>PPGP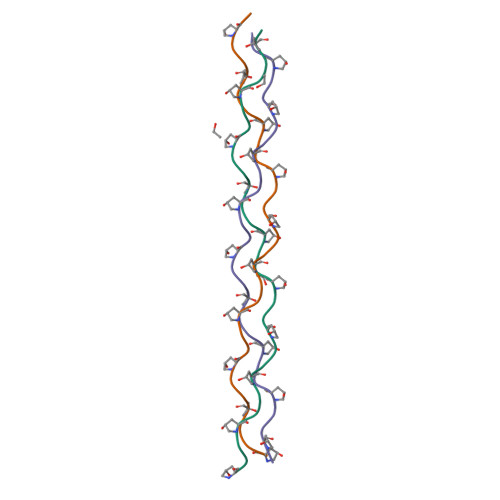PGPPGPPGLPGPPGPPGPPGPPGPPG[3x]> MSVGLIAPLASPIQESRANTNIENIGDGAEVIKRTEDVSSK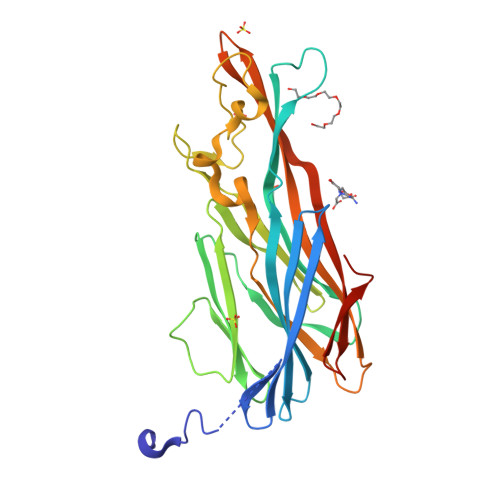KWGVTQNVQFDFVKDKKYNKDALIVKMQGFINSRTSFSDVKGSGYELTKRMIWPFQYNIGLTTKDPNVSLINYLPKNKIETTDVGQTLGYNIGGNFQSAPSIGGNGSFNYSKTISYTQKSYVSEVDKQNSKSVKWGVKANEFVTPDGKKSAHDRYLFVQSPNGPTGSAREYFAPDNQLPPLVQSGFNPSFITTLSHEKGSSDTSEFEISYGRNLDITYATLFPRTGIYAERKHNAFVNRNFVVRYEVNWKTHEIKVKGHNKHHHHHH2,4-dimethyl-6-(piperazin-1-yl)pyrimidine | C10 H16 N4 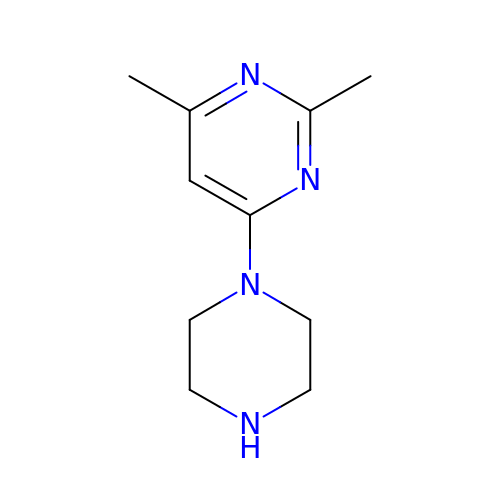| NARMKNJWXHFJFF-UHFFFAOYSA-N> KVEDPKDFPVDLHAFLSQAVFSNRTVASFAVYTTKEKAQILYKKLMEKYSVTFISRHGFGGHNILFFLTPHRHRVSAINNYCQKLCTFSFLICKGVNKEYLFYSALCRQPYAVVEESIQGGLKEHDLNPE

A conserved feature of Polyomavirus T-antigens is a phenylalanine situated at the C-termini of their origin-binding domains (OBDs). T-ag is the only virally encoded protein needed for replication; therefore, it has been the target of numerous studies designed to understand its multiple roles during the duplication of the viral genome. One of the interesting findings of the JCV T-ag OBD structure was the presence of a C-terminal "pocket". This structure also revealed that the pocket serves as the binding site for T-ag residues from the A1/B2 loops situated on a neighboring OBD subunit. The initial function of the A1 and B2 loops is site-specific DNA binding to the viral origin.

JCV T-ag containing the F258L mutation, which is located in the C-terminus of the OBD, was unable to support T-ag dependent JCV DNA replication. The F258L JCV T-ag OBD crystallized in the I41 space group, diffracted to 2.7 Å and contained one molecule in the asymmetric unit cell. As with the wt JCV OBD, the topology of the OBD F258L mutant is a five-stranded antiparallel B-sheet sandwiched, on either side, by two helices. The A1 loop is the "DNA free" or "apo-conformation" (; reviewed in [26]). Inspection of Fig 4B establishes that the previously described C-terminal pocket is also a feature of the JCV T-ag OBD F258L mutant. The crystallography experiments establish that the overall structures of the apo forms of the wt and F258L JCV T-ag OBDs are quite similar and that the structural consequences of the F258L mutation appear to be localized to the pocket. For example, the H-bond formed between N259 and R155 is lost and many non-bonded interactions made between the C-terminus and the A1 and B2 motifs are altered. Moreover, L258 causes disruptions to many of the non-bonded interactions and the L258 mutation also causes the loss (e.g., N259-R155) and acquisition (e.g., D257-F152) of several hydrogen bonds. That the changes are localized to the pocket, and not transmitted to other regions of the JCV T-ag OBD, is supported by the observation that the F258L mutation has little to no impact on A1 and B2 loop dependent site-specific binding to duplex DNA.N-[(4-bromothiophen-2-yl)methyl]acetamide | C7 H8 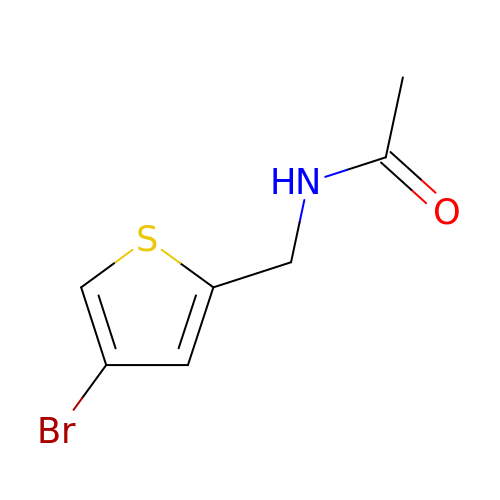Br N O S | GPLBTWBXJXXSBT-UHFFFAOYSA-N> NSELDRLSKDDRNWVMQTKDYSATHFSRLTEINSHNVKNLKVAWTLSTGTLHGHEGAPLVVDGIMYIHTPFPNNVYAVDLNDTRKMLWQYKPKQNPAARAVACCDVVNRGLAYVPAGEHGPAKIFLNQLDGHIVALNAKTGEEIWKMENSDIAMGSTLTGAPFVVKDKVLVGSAGAELGVRGYVTAYNIKDGKQEWRAYATGPDEDLLLDKDFNKDNPHYGQFGLGLSTWEGDAWKIGGGTNWGWYAYDPKL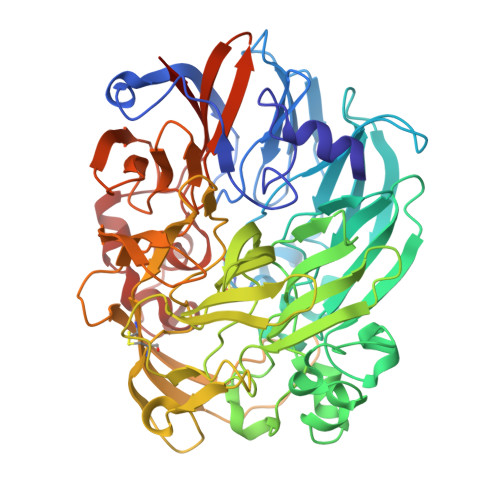DMIYYGSGNPAPWNETMRPGDNKWTMTIWGRDADTGRAKFGYQKTPHDEWDYAGVNYMGLSEQEVDGKLTPLLTHPDRNGLVYTLNRETGALVNAFKIDDTVNWVKKVDLKTGLPIRDPEYSTRMDHNAKGICPSAMGYHNQGIESYDPDKKLFFMGVNHICMDWEPFMLPYRAGQFFVGATLNMYPGPKGMLGQVKAMNAVTGKMEWEVPEKFAVWGGTLATAGDLVFYGTLDGFIKARDTRTGELKWQFQLPSGVIGHPITYQHNGKQYIAIYSGVGGWPGVGLVFDLKDPTAGLGAVGAFRELAHYTQMGGSVFVFSL>MDLKPDNYFSGQQLTLARAIENGEVDEVIKLASGTDLNKPGKEDMTLLFWAVMNSINNQKTPERLNVITMLIKAGADPLQPRPQGKNSPAEFVLMADNADWIKAMLNAGLSPNAVDKTFGKPIIFQTLEAKNTKTLQAMLDKGADINITDSLGNTLLIDALDFHSYDHVLLLLERGADPEIKADNGWTMGNQLQRFLDRAKVGSDEYKKLNEIKDVLIQHGGKWPPTPVK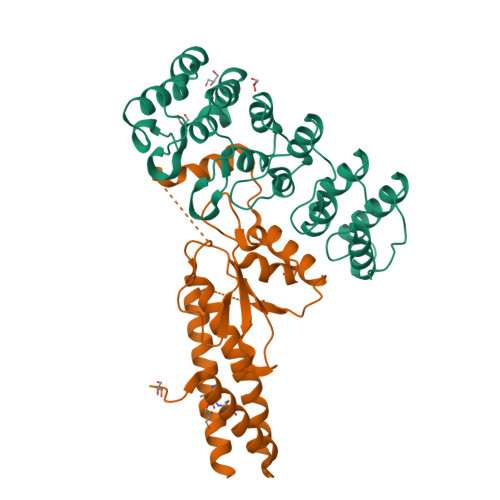[2x];>[2x]MAKSHHHHHHTSTKAERWQARKDLIAKGSNSLYPDAQIAAKRLAANNIAVEKAKLAENVYKTVNPLEATPGVPEGWKDISNDAGALKKYGLDKEVLFDHADTPDFLARVYQPDSAVFGSDMNPTIVFRGSRQPEFFPTKNMADWINNGAQGLGMESDYYKRAVRLGSRLAKSVSKIDIAGHSLGGGLASATSIASGQAGWTFNAAGLHSTTVEKYGGSLLGEADNIQAYRVEGELLTKIQEVNLAEDYKMLKGHIPTLIAKEEISAIMPNAAGVVHDLPGGTGGPLDRHGIGQAIDCIEQQKDEDISIIRSRA Binding of human norovirus to histo blood group antigens (HBGAs), a critical step preceding host-cell entry, has been the focus of a substantial number of biophysical studies involving nuclear magnetic resonance (NMR) experiments, native mass spectrometry (MS), surface plasmon resonance, or crystallography as this has been reviewed recently. The highly conserved HBGA-binding sites are located in the P2 subdomain of the P-domain of the norovirus capsid protein VP116–18. Here, we present an almost complete backbone assignment of the P-dimers and uncover spontaneous deamidation of asparagine 373, influencing HBGA binding. In the assignment process we discovered that N373, located in a loop directly adjoining the HBGA-binding site, transforms into an iso-aspartate, isoD373, within 1–2 days at body temperature.

The deamidated form of Saga P-dimers was then subjected to crystal structure analysis in the presence of methyl α-l-fucopyranoside. Well-diffracting apo crystals were obtained belonging to the space group P21, different from C21 as observed previously for the native form of Saga P-dimers. Upon incubation of deamidated P-dimer apo crystals with 600 mM methyl α-l-fucopyranoside we obtained a co-crystal structure at 1.52 Å resolution, in which the isoD373 isopeptide bond is clearly visible in one of the two protein chains that comprise the asymmetric unit (i.e. in one half of the P-dimer). We also observed binding of methyl α-l-fucopyranoside to the two canonical HBGA-binding sites in the Saga P-dimer. In the chain with unambiguous density for the isopeptide bond the side chain of D374 is rotated such that one oxygen of the γ-carboxy group forms a single hydrogen bond to OH-4 of methyl α-l-fucopyranoside (left). In this chain, no unambiguous density is observed for residue 373 and the preceding amino acids, and so the density does not allow us to determine whether this chain contains an N373 or an isoD373 residue. In our crystal structure of the deamidated P-dimer complexed with methyl α-l-fucopyranoside two binding geometries can be observed at the same time, i.e. one in each crystallographically distinct half of the P-dimer. Fucose binds to the modified binding pocket in much the same place and orientation as observed for the native protein, but the hydrogen bonding to the side chain carboxy group of D374 appears altered as shown in Fig. 7 and Supplementary Fig. 23. The altered D374 side-chain orientation and the loss of one hydrogen bond can be explained by altered conformational dynamics of the loop. Except for the loop carrying the isopeptide bond, the overall structure of the P-dimers is very similar to the structures published before.

>TGSKPFTVPILTVEEMTNSRFPIPLEKLFTGPSGAFVVQPQNGRCTTDGVLLGTTQLSPVNICTFRGDVTHIAGSRNYTMNLASLNWNNYDPTEEIPAPLGTPDFVGKIQGLLTQTTKGDGSTRGHKATVYTGSAPFTPKLGSVQFSTDTEDDFETHQNTKFTPVGVIQDGSTTHRNEPQQWVLPSYSGRNVHNVHLAPAVAPTFPGEQLLFFRSTMPGCSGYPNMDLDCLLPQEWVQHFYQEAAPAQSDVALLRFVNPDTGRVLFECKLHKSGYVTVAHTGQHDLVIPPNGYFRFDSWVNQFYTLAPM[2x]Amongst the Arabidopsis MSL channels, MSL10 is enigmatic in that it has two separable functional modalities, regulated cell death signaling conferred by its N-terminal soluble ‘death’ domain and force-activated ion channel activity imparted by its C-terminal portion. When heterologously expressed in Xenopus oocytes, MSL10 is indeed activated by membrane stretch and displays a preference for anions. In Arabidopsis, MSL10 is primarily expressed in the shoot apex, root tips, and vascular tissues, playing a critical role in adaptation to hypo-osmotic shock and induction of programmed cell death. Analogous to DmMSL10/FLYC1, each subunit of the heptameric AtMSL10 channel is composed of a transmembrane domain (TMD) with six membrane-spanning helices (TM1-TM6) and a characteristic C-terminal cytoplasmic domain (CTD) shared by all MscS homologs.

We expressed the full-length wild-type AtMSL10 channel, consisting of 734 amino acids, in Pichia pastoris and purified the channel to homogeneity for single-particle cryo-EM analysis. The channel core, consisting of TM3-TM6 and the cytoplasmic C-terminal domain, was well resolved in the cryo-EM density map and allowed unambiguous placement of most of the side chains. However, the N-terminal ‘death’ domain (residues 1–165), part of the cytoplasmic domain between TM4 and TM5, including residues 335–386, 397–431, and 469–480, and the C-terminal end (residues 732–734), were not resolved in the reconstruction, and thus were absent in the final refined atomic model. AtMSL10 assembles as a symmetric heptamer in that the cryo-EM reconstructions without applied symmetry (C1 symmetry) and with imposed C7 symmetry are essentially identical. In contrast, reconstructions of AtMSL10 in C1 or C7 symmetry indicated that all CLDs adopt the ‘down’ configuration. To evaluate the conformational state of the wild-type AtMSL10 structure, we calculated the pore radius using program HOLE36. Strikingly, pore radius estimation indicated a wide-open central ion conduction path. In contrast, the wild-type DmMSL10/FLYC1 channel, which is the closest ortholog of AtMSL10, has a minimum radius of 3.5 Å at the equivalent hydrophobic gate. Thus, comparison of the ion-conduction pore dimensions of these channels indicates that the AtMSL10 structure likely represents an open conformation, which is remarkable because the wild-type AtMSL10 structure was determined in the absence of applied membrane tension that is required for channel activation. The open AtMSL10 structure was determined in detergent micelles that were essentially devoid of membrane lipids. Consistently, we did not observe lipid-like densities surrounding the channel.

>[7x]MAEQKSSNGGGGGGDVVINVPVEEASRRSKEMASPESEKGVPFSKSPSPEISKLVGSPNKPPRAPNQNNVGLTQRKSFARSVYSKPKSRFVDPSCPVDTSILEEEVREQLGAGFSFSRASPNNKSNRSVGSPAPVTPSKVVVEKDEDEEIYKKVKLNREMRSKISTLALIESAFFVVILSALVASLTINVLKHHTFWGLEVWKWCVLVMVIFSGMLVTNWFMRLIVFLIETNFLLRRKVLYFVHGLKKSVQVFIWLCLILVAWILLFNHDVKRSPAATKVLKCITRTLISILTGAFFWLVKTLLLKILAANFNVNNFFDRIQDSVFHQYVLQTLSGLPLMEEAERVGREPSTGHLSFATVVKKGTVKEKKVIDMGKVHKMKREKVSAWTMRVLMEAVRTSGLSTISDTLDETAYGEGKEQADREITSEMEALAAAYHVFRNVAQPFFNYIEEEDLLRFMIKEEVDLVFPLFDGAAETGRITRKAFTEWVVKVYTSRRALAHSLNDTKTAVKQLNKLVTAILMVVTVVIWLLLLEVATTKVLLFFSTQLVALAFIIGSTCKNLFESIVFVFVMHPYDVGDRCVVDGVAMLVEEMNLLTTVFLKLNNEKVYYPNAVLATKPISNYFRSPNMGETVEFSISFSTPVSKIAHLKERIAEYLEQNPQHWAPVHSVVVKEIENMNKLKMALYSDHTITFQENRERNLRRTELSLAIKRMLEDLHIDYTLLPQDINLTKKNSLEVLFQ> GPLGSDVKDHKLLLFQEVTGLISTWVTSIVEEADWDFERALKLFIQKNADHEIPDLAFAGSGSGSGSLSKADKRSLAVARAEL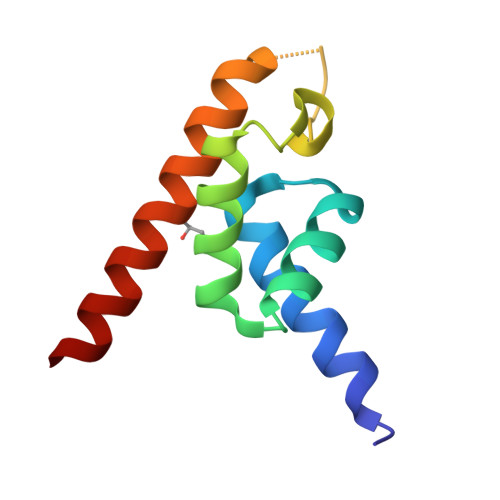VLEQIQQKANK>[3x]MDFLSNFLTDFVGQLQSPTLAFLIGGMVIAALGTQLVIPEAISTIIVFMLLTKIGLTGGMAIRNSNLTEMLLPVAFSVILGILIVFIARFTLAKLPNVRTVDALATGGLFGAVSGSTMAAALTTLEESKISYEAWAGALYPFMDIPALVTAIVVANIYLNKRKRKSAAASIEESFSKQPVAAGDYGDQTDYPRTRQEYLS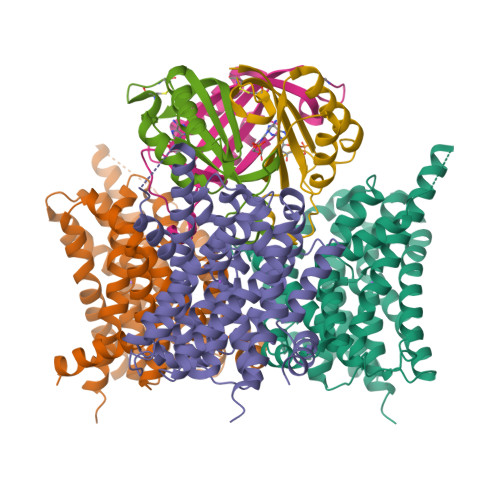QQEPEDNRVKIWPIIEESLQGPALSAMLLGLALGIFTKPESVYEGFYDPLFRGLLSILMLIMGMEAWSRIGELRKVAQWYVVYSLIAPIVHGFIAFGLGMIAHYATGFSLGGVVVLAVIAASSSDISGPPTLRAGIPSANPSAYIGSSTAIGTPIAIGVCIPLFIGLAQTLGAG;>[3x]MAKPANKLVIVTEKILLKKIAKIIDESGAKGYTVMNTGGKGSRNVRSSGQPNTSDIEANIKFEILTETREMAEEIADRVAVKYFNDYAGIIYICSAEVLYGHTFCGPEGC>[2x]MGSSHHHHHHHHHHSSGLVPRGSHMTGHSNGQDLVMKANEKYLVKNAQQPERGKIYDRNGKVLAEDVERYKLVAVIDKKASANSKKPRHVVDKKETAKKLSTVIDMKPEEIEKRLSQKKAFQIEFGRKGTNLTYQDKLKIEKMNLPGISLLPETERFYPNGNFASHLIGRAQKNPDTGELKGALGVEKIFDSYLSGSKGSLRYIHDIWGYIAPNTKKEKQPKRGDDVHLTIDSNIQVFVEEALDGMVERYQPKDLFAVVMDAKTGEILAYSQRPTFNPETGKDFGKKWANDLYQNTYEPGSTFKSYGLAAAIQEGAFDPDKKYKSGHRDIMGSRISDWNRV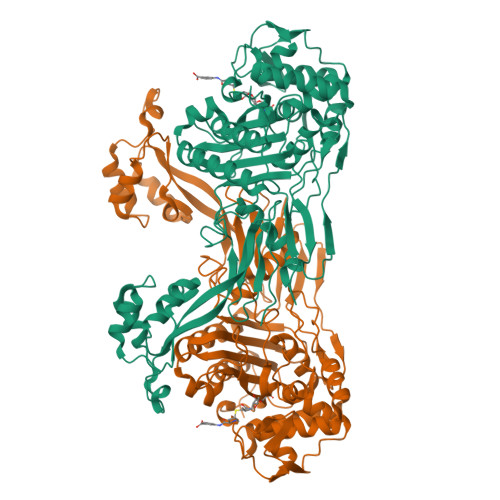GWGEIPMSLGFTYSSNTLMMHLQDLVGADKMKSWYERFGFGKSTKGMFDGEAPGQIGWSNELQQKTSSFGQSTTVTPVQMLQAQSAFFNDGNMLKPWFVNSVENPVSKRQFYKGQKQIAGKPITKDTAEKVEKQLDLVVNSKKSHAANYRIDGYEVEGKTGTAQVAAPNGGGYVKGPNPYFVSFMGDAPKKNPKVIVYAGMSLAQKNDQEAYELGVSKAFKPIMENTLKYLNVGKSKDDTSNAEYSKVPDVEGQ> MDLEMMLDEDYKEGICLIDFSQIALSTALVNFPDKEKINLSMVRHLILNSIKFNVKKAKTLGYTKIVLCIDNAKSGYWRRDFAYYYKKNRGKAREESTWDWEGYFESSHKVIDELKAYMPYIVMDIDK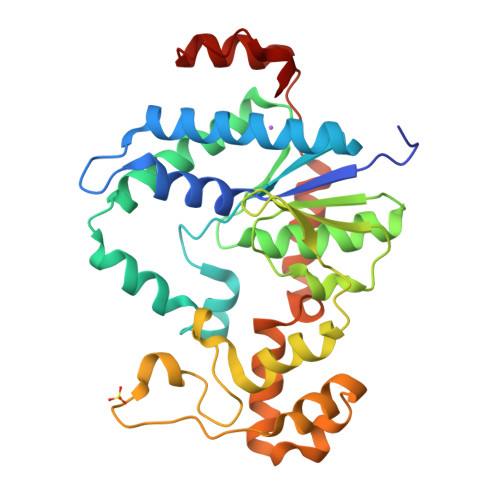YEADDHIAVLVKKFSLEGHKILIISSDGDFTQLHKYPNVKQWSPMHKKWVKIKSGSAEIDCMTKILKGDKKDNVASVKVRSDFWFTRVEGERTPSMKTSIVEAIANDREQAKVLLTESEYNRYKENLVLIDFDYIPDNIASNIVNYYNSYKLPPRGKIYSYFVKAGLSKLTNSINEF> MSHGASSRPATARKSSGLSGTVRIPGDKSISHRSFMFGGLASGETRITGLLEGEDVINTGKAMQAMGARIRKEGDTWIIDGVGNGGLLAPEAPLDFGNAATGCRLTMGLVGVYDFDSTFIGDASLTKRPMGRVLNPLREMGVQVKSEDGDRLPVTLRGPKTPTPITYRVPMASAQVKSAVLLAGLNTPGITTVIEPIMTRDHTEKMLQGFGANLTVETDADGVRTIRLEGRGKLTGQVIDVPGDPSSTAFPLVAALLVPGSDVTILNVLMNPTRTGLILTLQEMGADIEVINPRLAGGEDVADLRVRSSTLKGVTVPEDRAPSMIDEYPI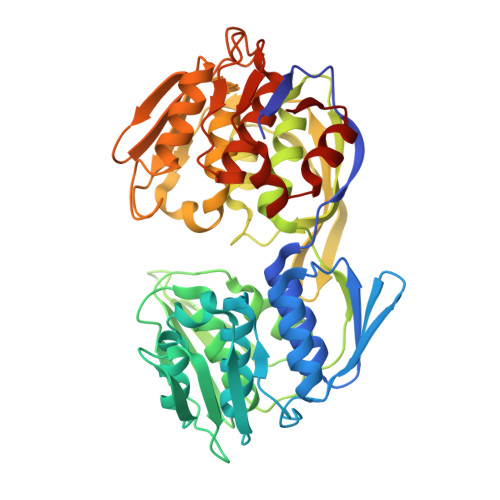LAVAAAFAEGATVMNGLEELRVKESDRLSAVANGLKLNGVDCDEGETSLVVRGRPDGKGLGNASGAAVATHLDHRIAMSFLVMGLVSENPVTVDDATMIATSFPEFMDLMAGLGAKIELSDTKAA(2E)-N-[(1,2-dimethyl-1H-indol-3-yl)methyl]-N-methyl-3-(7-oxo-5,6,7,8-tetrahydro-1,8-naphthyridin-3-yl)prop-2-enamide | C23 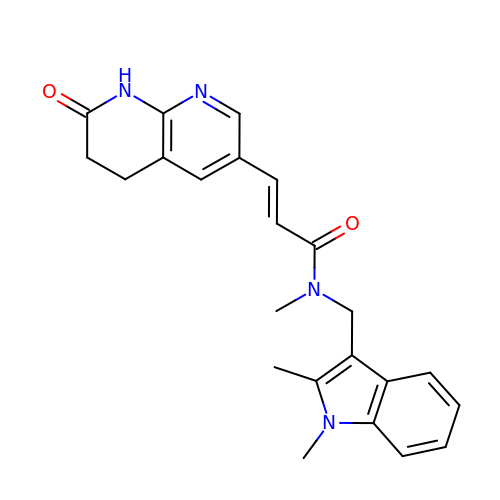H24 N4 O2 | PVNPCRMKZHRPEV-DHZHZOJOSA-N>SNAMKTYDYIVIGGGSGGIASANRAGMHGANVLLIEGNEIGGTCVNVGCVPKKVMWQASSMMEMMERDTAGYGFDVEIKNFSFKQLVENREKYIDFLHGAYNRGLDSNNIERIHGYATFTGEQTIEVNGTEYTAPHILIATGGRPKKLGIPGEEYALDSNGFFALEEMPKRVVFVGAGYIAAELAGTLHGLGAETHWAFRHERPLRSFDDMLSEKVVERYQEMGMQIHPNATPAKIEKTAQNEYVITFENGESITTDAVIFGTGRQPNTDQLGLENTKVALDEKGYVKVDKFQNTTQNGIYAVGDVIGKIDLTPVAIAAGRRLSERLFNGQTDLYLDYNLVP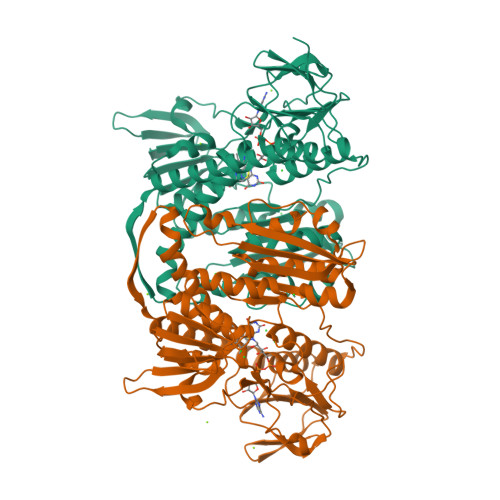TVVFTHPPVATIGLTEKAALEEYGEDQVKIYRSSFTPMYFALGEYRQKCDMKLICVGKEEKIVGLHGIGIGVDEMLQGFAVAIKMGATKADFDNTVAIHPTGSEEFVTMR[4x]>[6x]MAKTIHTDKAPAAIGPYVQGKIVGNLLFASGQIPLSPETGEIIGTTIEEQTQQVLKNVSAILEAAGTDFDHVVKATCFLSDINDFVAFNEVYKTAFTEAFPARSAVEVARLPKDVKIEIEV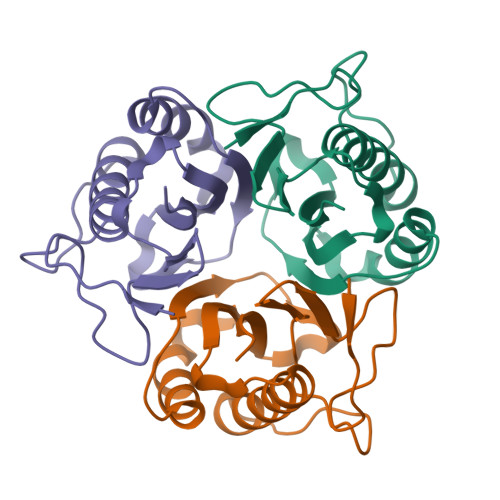IAEIL> GNYKKPKLLYCSNGGHFLRILP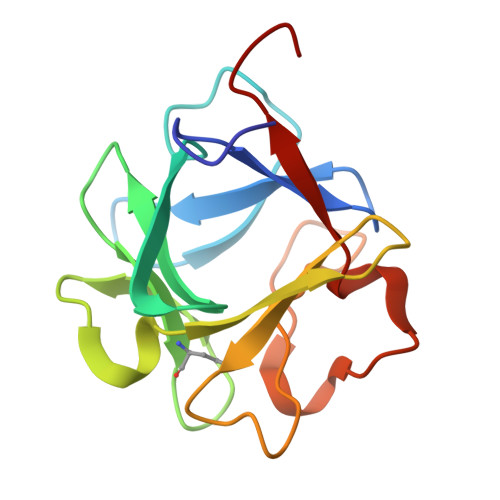DGTVDGTRDRSDQHIQLQLSAESVGEVYIKSTETGQYLAMDTDGLLYGSQTPNEECLFLERLEENHYNTYISKKHAEKNWFVGLKKNGSCKRGPRTHYGQKAILFLPLPVSSD> CVICDPSVVLALKSLEKDYLPGHLDAKHHKAMMERVENAVKDFQELSLNEDAYMGVVDEATLQKGSWSLLKDLKRITDSDVKGDLFVKELFWMLHLQKETFATYVARFQKEAYCPNKCGVMLQTLIWCKNCKKEVHACRKSYDCGERNVEVPQMEDMILDCELNWHQASEGLTDYSFYRVWGNNTETLVSKGKEATLTKPMVGPEDAGSYRCELGSVNSSPATIINFHVTVLPGRAVPR;> GDELLNICMNAKHHKRVPSPEDKLYEECIPWKDNACCTLTTSWEAHLDVSPLYN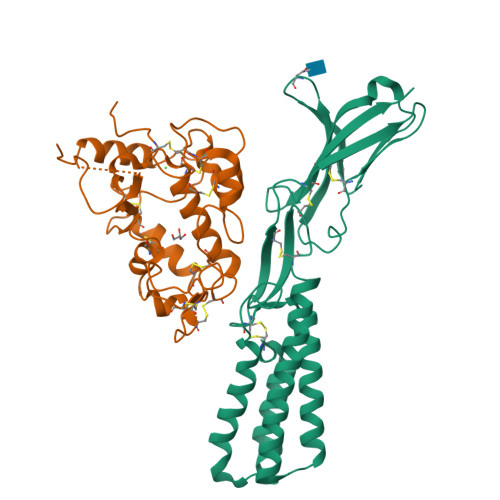FSLFHCGLLMPGCRKHFIQAICFYECSPNLGPWIQPVGSLGWEVAPSGQGERVVNVPLCQEDCEEWWEDCRMSYTCKSNWRGGWDWSQGKNRCPKGAQCLPFSHYFPTPADLCEKTWSNSFKASPERRNSGRCLQKWFEPAQGNPNVAVARLFASGRLVPR> MAIETNAVVITDLNPLYPRDRDYIYEGAAQIRLIKQ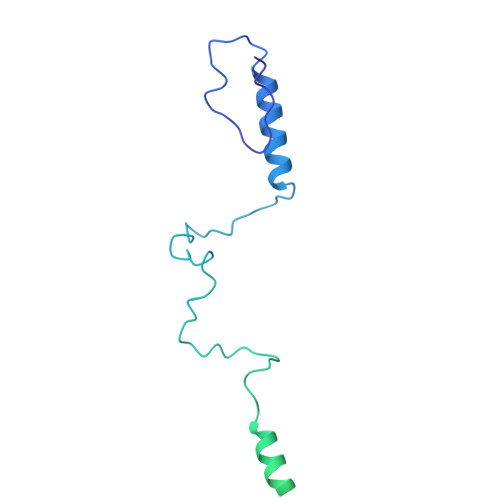TLQNTFPNVTEPVDIDSDTFKIMSEKLKFTGDAMDVGGLMIKNVTPGTGDKDVVTKGQMEAFMKNWMENKLYRIGSYYITEEDINPGDSISLGFGSWAKVTGVIMGTGVVNPDGSVPNAQRVEFQAGGTGGRVFNTIRTENVPLMTVNGSSFSLSSNTHSHNMVFGRGDASGHNSSPNWYSPGGGYSQRTDNDTHTHTISGSVSLGRDDISRQPINTLPPFRAAHIWRRIS>GSHMKNSVSVDLPGSMKVLVSKSSNADGKYDLIATVDALELSGTSDKNNGSGVLEGVKADASKVKLTISDDLGQTTLEVFKSDGSTLVSKKVTSKDKSSTFELFNEKGELSFKLITRADKSSTFELFNEKGELSFKLITRADKSSTFELFNEKGELSFKLITRADKSSTFELFNEKGELSFKLITRADGTRLEYTGIKSDGSGKAKEVLKGYVLEGTLTAEKTTLVVKEGTVTLSKNISKSGEVSVELNDTDSSAATKKTAAWNSGTSTLTITVNSKKTKDLVFTSSNTITVQQYDSNGTSLEGSAVEITKL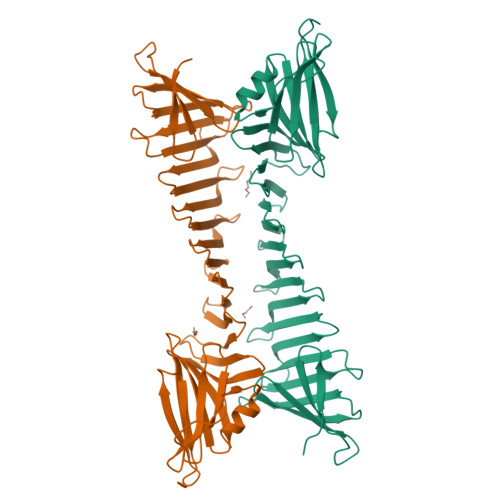DEIKNALK[2x]>[4x]MRFTILSVLAFSLPLVLAETPAPSCPVTNVTTPQLDPITQAYADAISSRPSLFAFPLPEIRDGYQSNVSDPSTEFTTKILSLPVGPTGNVTAYLYKPVSGEREKGKDLLPVIAYFHGGGWVFGGPKSYRGLITNL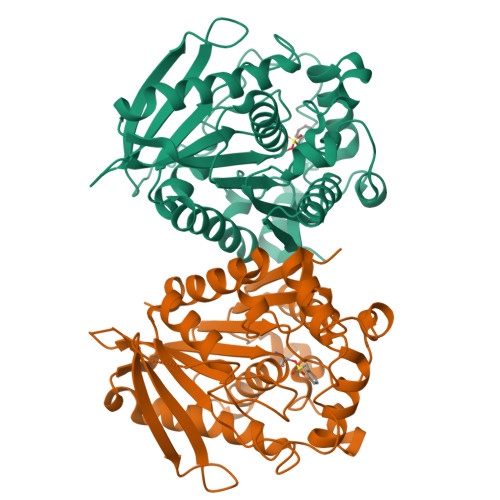IRESGAAVFFVDYTLTPKVAYPVPNEQCYAAVQWLLEHGEKLGVDPTNMGFGGDSAGGELSSSVSLLSIKRKTPLPKFQVLIYPATDLACESATFKEFPNGPGLTTDEIRFAASLFTPDPKSRLEDVASPGRASDEDLAKFPETLIVVAEVDPIRQQGEDFGRRLQKLGVRAAIIRVLGTIHGFASIDVLSEAPGAKATIELIGYKFKKALH>[3x]MGDIQVQVNIDDNGKNFDYTYTVTTESELQKVLNELMDYIKKQGAKRVRISITARSSKEAYKFLAILAKVFAELGYNDINRKMTVRFRGDDLEALEKALKEMIRQARKFAGTVTYTLDGNDLEITITGVPRQVLEELAKEAERLAKEFNITITITVTVEGQLGSLEHHHHHH

Here, we explore the viability of such a mechanism by inserting one de novo designed alpha beta protein into another such that the two beta sheets are combined into one. The backbone geometry at the junctions between the original domains is regularized, and the sequence at the newly formed interface is optimized to stabilize the single integrated domain structure. Crystal structures of two such proteins demonstrate that complex beta sheet structures can be designed with considerable accuracy using this approach and provide a proof-of-concept for the hypothesis that complex beta topologies in natural proteins may have evolved from simpler beta sheet structures in a similar manner. Our success in designing larger beta sheet domains by recombining smaller independently folded beta sheet proteins suggests a similar mechanism could have played a role in the evolution of naturally occurring complex beta sheet proteins.

A first extended sheet protein was created by inserting a designed ferredoxin domain into a beta turn of the designed TOP7 protein to create a half-barrel structure, with the two sheets fused into a single seven strand sheet flanked by four helices. The CD spectra show both alpha and beta structures. The most similar SCOP domains had weak TM-align scores (0.54 and 0.51), and the sheets in these matched structures have different connectivities than those of the designs, suggesting that the two designed proteins have novel folds. The beta strand connectivity is quite different in the designs than in these closest structural matches.> MATISNLASDIQSQVDVIDSYLKKHNLQQPSFEVDSPSELPLDANVQRARLKLIETATSLANLAIGSADHLRWHCMNNKYDDMVLHFLARYNIFDAVPRNESISYVELSQKIGLPEHRLRRIMSM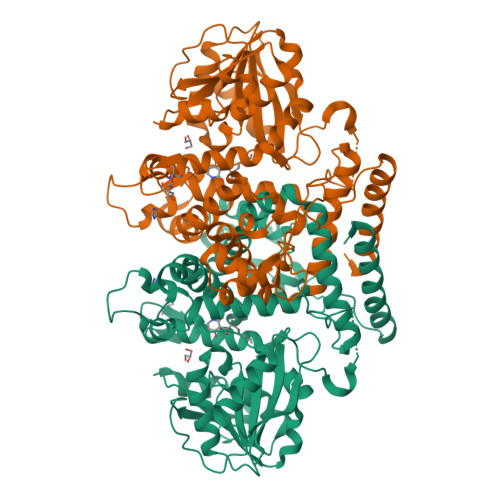AYTRHLFCEPKPGFVAHTSNSALAINDPLAMAWILHNVEEVQPWYANKLVDSTKKWGDTTDPRHTGPNLNAKAGEEKLFYQIMEEDDQGEWNGVKGKGFRLWRLFDTDKFFGTGGAIKGTNMLRAFDWGKLGKATVVDLSGITGHLSSTVALAYPDLTFIVQERNQSWLEKQFNDKLPAELKGSGRVRFMAHDKYAQQPVKDVDVFFMSTMLHKEPDEKAITILRHCAEAMDPKKSRIVTRDIVLDGGDPPAEDALESGKGINGKNEVYQAGLGPTGVITRLNAGIDLQMLAVLNAFERTREDWITLFKTADPRFVLKACIQTVGDCASVMEWVLEEE>[2x]GAMTKPRFTTGLVYDTLMLKHQCTAGSSSSHPEHAGRIQSIW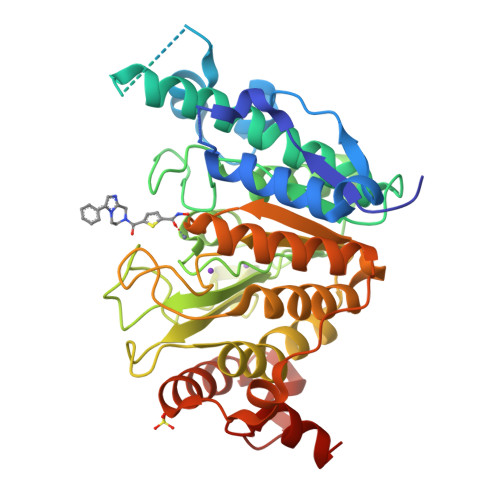SRLQETGLRGKCEAIRGRKATLEELQTVHSEAHTLLYGTNPLNRQKLDSKKLLGSLASVFVRLPCGGVGVDSDTIWNEVHSAGAARLAVGCVVELVFKVATGELKNGFAVVRPPGHHAEESTPMGFCYFNSVAVAAKLLQQRLSVSKILIVDWDVHHGNGTQQAFYSDPSVLYMSLHRYDDGNFFPGSGAPDEVGTGPGVGFNVNMAFTGGLDPPMGDAEYLAAFRTVVMPIASEFAPDVVLVSSGFDAVEGHPTPLGGYNLSARCFGYLTKQLMGLAGGRIVLALEGGYDLTAICDASEACVSALLGNELDPLPEKVLQQRPNANAVRSMEKVMEIHSKYWRCLQRTTSTAGRSLIEAQTCENEEAETVT N-benzyl-2-(cyclohex-1-en-1-yl)ethan-1-amine | 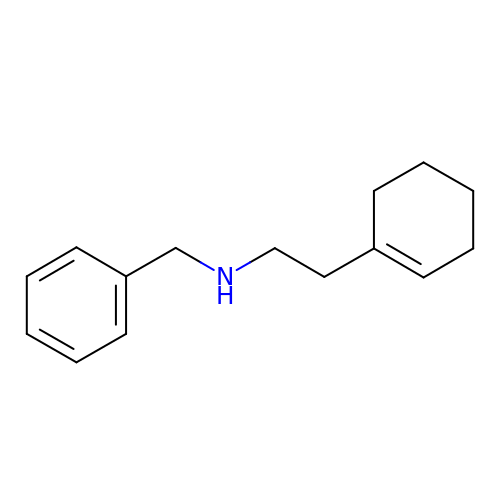C15 H21 N | RTJNHLXWVAXRBH-UHFFFAOYSA-N>[900x]MADVTGIALGMIETRGLVPAIEAADAMTKAAEVRLVGRQFVGGGYVTVLVRGETGAVNAAVRAGADACERVGDGLVAAHIIARVHSEVENILPKAPQA;>[60x]M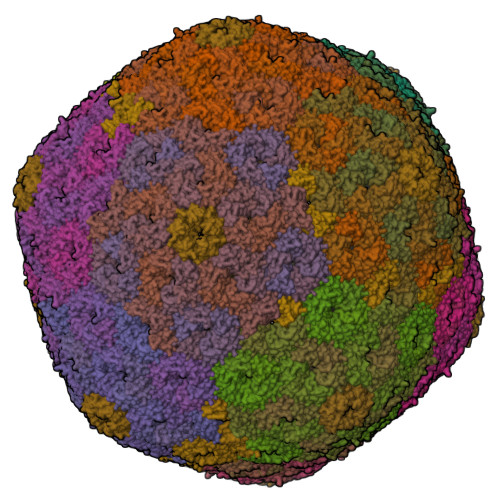KIMQVEKTLVSTNRIADMGHKPLLVVWEKPGAPRQVAVDAIGCIPGDWVLCVGSSAAREAAGSKSYPSDLTIIGIIDQWNGE;>MPSQSGMNPADLSGLSGKELARARRAALSKQGKAAVSNKTASVNRSTKQAASSINTNQVRSSVNEVPTDYQMADQLCSTIDHADFGTESNRVRDLCRQRREALSTIGKKAAKTTGKPSGRVRPQQSVVHNDAMIENAGDTNQSSSTSLNNELSEICSIADDMPERFGSQAKTVRDICRARRQALSERGTRAVPPKPQSQGGPGRNGYQIDGYLDTALHGRDAAKRHREMLCQYGRGTAPSCKPTGRVKNSVQSGNAAPKKVETGHTLSGGSVTGTQVDRKSHVTGNEPGTCRAVTGTEYVGTEQFTSFCNTSPKPNATKVNVTTTARGRPVSGTEVSRTEKVTGNESGVCRNVTGTEYMSNEAHFSLCGTAAKPSQADKVMFGATARTHQVVSGSDEFRPSSVTGNESGAKRTITGSQYADEGLARLTINGAPAKVARTHTFAGSDVTGTEIGRSTRVTGDESGSCRSISGTEYLSNEQFQSFCDTKPQRSPFKVGQDRTNKGQSVTGNLVDRSELVTGNEPGSCSRVTGSQYGQSKICGGGVGKVRSMRTLRGTSVSGQQLDHAPKMSGDERGGCMPVTGNEYYGREHFEPFCTSTPEPEAQSTEQSLTCEGQIISGTSVDASDLVTGNEIGEQQLISGDAYVGAQQTGCLPTSPRFNQTGNVQSMGFKNTNQPEQNFAPGEVMPTDFSIQTPARSAQNRITGNDIAPSGRITGPGMLATGLITGTPEFRHAARELVGSPQPMAMAMANRNKAAQAPVVQPEVVATQEKPELVCAPRSDQMDRVSGEGKERCHITGDDWSVNKHITGTAGQWASGRNPSMRGNARVVETSAFANRNVPKPEKPGSKITGSSGNDTQGSLITYSGGARG[120x]> GHMGNRTFSYTLEDHTKQAFGIMNELRLSQQLCDVTLQVKYQD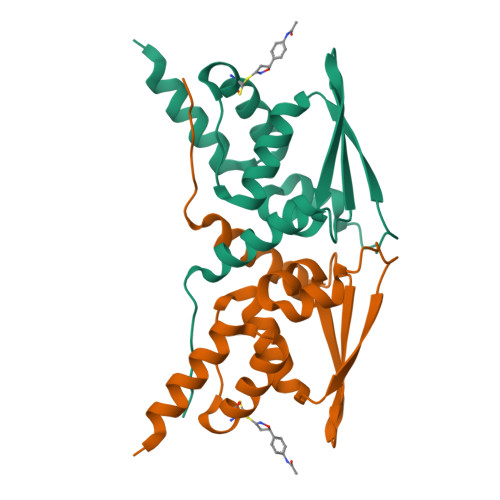APAAQFMAHKVVLASSSPVFKAMFTNGLREQGMEVVSIEGIHPKVMERLIEFAYTASISMGEKCVLHVMNGAVMYQIDSVVRACADFLVQQLD> GSHMAVEVCVKAAVGAPDILGDCPFSQRVLLTLEEKKITYEMKLVDLSNKPEWFLKISPEGKVPVFNSGDGKWIADSDVITQVIEEKFPTPSLVTPPEYASVGSKIFPSFVKFLKSKDASDGSEKALLDELQALDEHLKAHGPYISGENVSAADLSLGPKLFHLQVALEHFKGWKIPE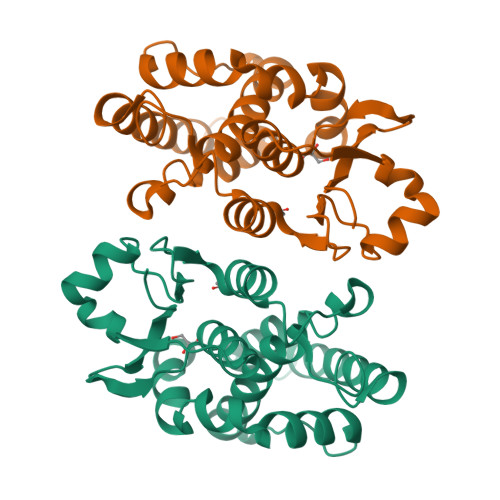NLTSVHAYTKALFSRESFVKTKPANQYLIAGWAPKVNA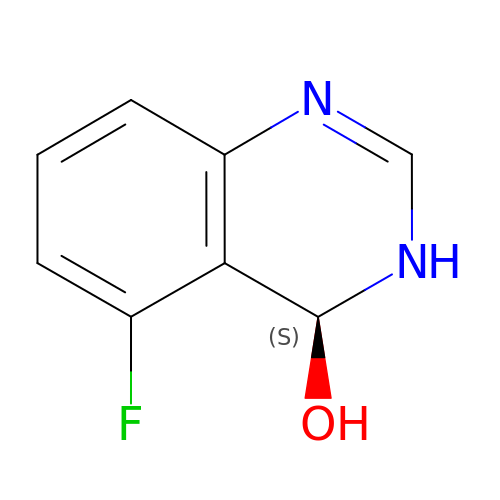5-fluoranyl-3,4-dihydroquinazolin-4-ol | C8 H7 F N2 O | VBPXEKJPOHSJCA-QMMMGPOBSA-N>MTNHIKEINWEQNTNSYIQLIPNIEYTKVEDTSLTLHLLVYRNPMDALFNRKGNQETYPLIIYLQGCGWGWTKQDTSAFIPQLVPFVEQGYVVASVQYRGSGEAVFPAQLHDVKTAVRFLKANAARYNIDPDRVGVWGDSSGGHLALLLGL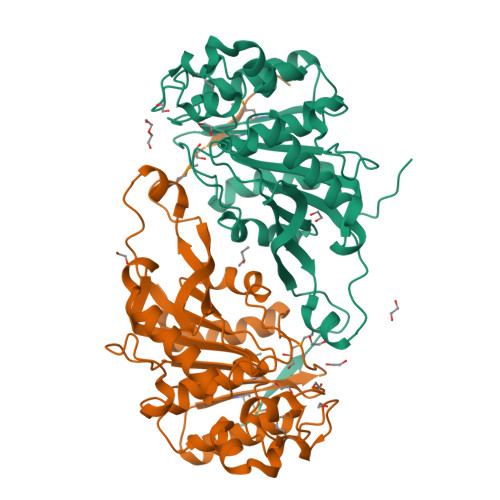TEGIEEFEGPDEYRHVSSKVDAVADWFGPVDLLSMSKYPSIFDHDSPNSPESKLIGGAVQENRVQAKQASPISYVHREAPPILIMHGDQDDVVPYQQSVQLFEALIKEGHDALMYKINGAGHNGFTQAHTLDIVKSFFRKHLKPGKAHHHHHH[4x]>[14x]MDMASRRKNARGLSGAVTALILVIASVIIALVVVGFAFG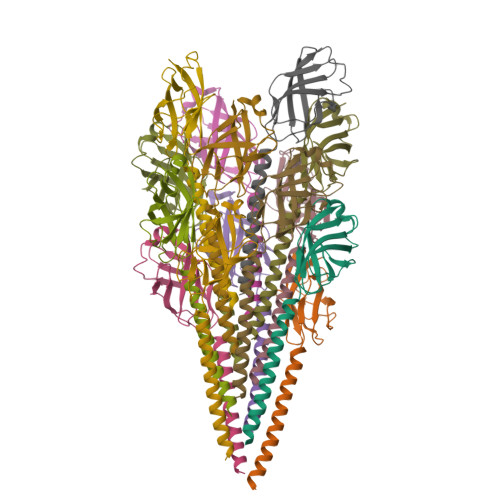LFGAFTGQGTVAQVGTATLSASTLTLTVTLKNTGASTQVTGVLINGNSGSVSGMTTISAGVNTYTITISIGSISTTLRGLVGSTISLTLILSNGETVTVSAIVTS>[6x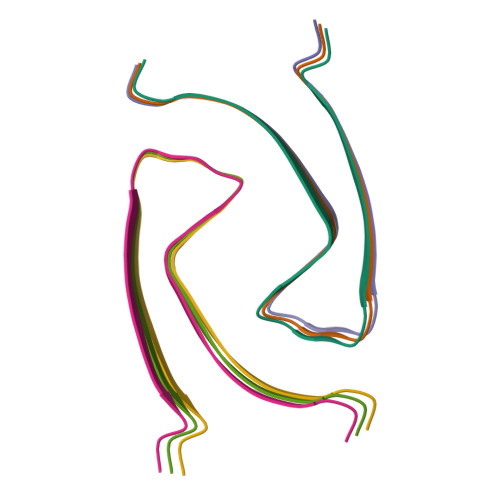]MPRGSRSAASRPASRPAAPSAHPPAHPPPSAAAPAPAPSGQPGLMAQMATTAAGVAVGSAVGHVMGSALTGAFSGGSSEPSQPAVQQAPTPAAPQPLQ> AERSELTIHPKEFTTFVRNFNPFLGATNLHTTTDF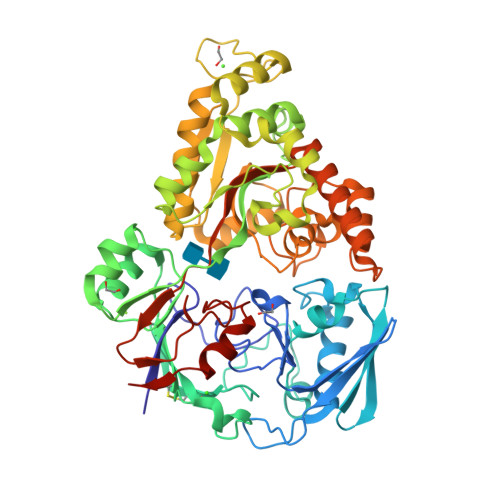IYEPLVVFNEMHGNTPVFRLAENFQMSDDLMSVTFDIRKGVKWSDGEAFTADDVVYSFNLVKEKPELDQSGINSWVTGVEKVNDYQVKFRLSEANSNVPYEIAKVPVVPKHVWSKVKDPSTFTNENPVGSGPFTVIDTFTPQLYIQCENPNYWDAANLDVDCLRVPQIANNDQFLGKVVNGEMDWTSSFVPDIDRTYAAASPKHHYWYPPAGTQAFVVNFKNPDAAKNEALTNVDFRRAFSMALDRQTIIDIAFYGGGTVNDFASGLGYAFEAWSDEKTHDKFKAYNSYNAEGAKKLLAKAGFKDVNKDGFVDTPSGKSFELLIQSPNGWTDFNNTVQLAVEQLAEVGIKARARTPDFSVYNQAMLEGTYDVAYTNYAHGADPYTYWNSAYNSALQSGDGMPRFAMHFYKNEKLDGLLNSFYKTADKQEQLEIAHGIQQIIAQDQVTIPVLSGAYMYQYNTTRFTGWWNEENPKGRPNIWAGIPERLLHVLDLKPVKHHHHHH>KNEPVLDTDGDELRAGEQYYVVSAIWGGGGGGLALGRLTNQQCPEIVVQRRSDLDNGIPVVFYNLDSNDDTVRVSTDLNVEFVPIRDRLCLTSTVWKVDNYDTSTGKWWVTTDGVIGNPGPHTLQSWFKIESGNLGYKFNFCPSVCESCITLCSDIGRYGNDGQMRLALAESGWPFV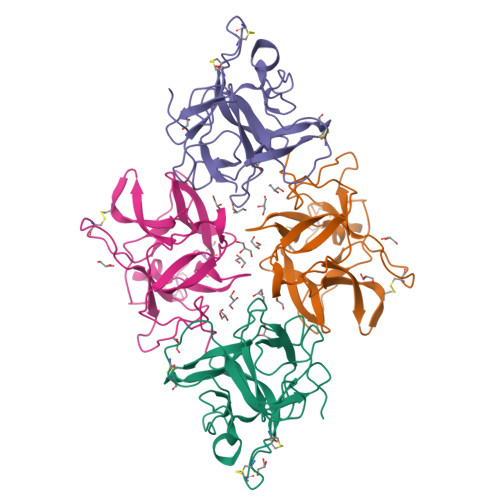FKKASSNIKQVVNAKH[4x]> MMEGVKDFKQELLLVLPA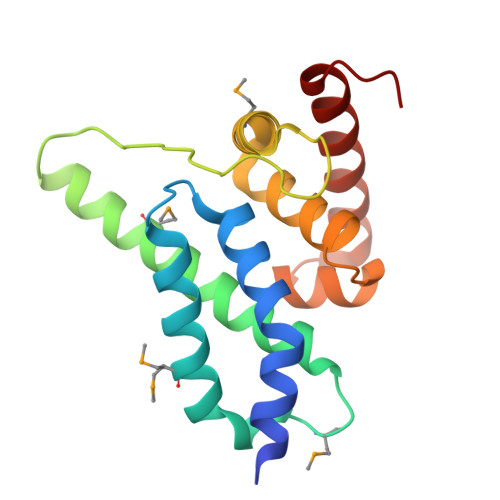LRAFAISLSSKHDKAEDLVQDTLMKAWAKQDSFEMGSNLKAWLFTILRNEFYSQMRKRGREVQDSDGVFIESVAIHPAQYGSLDLQDFKKALNMLSADQREAIILIGASGFSYEDAAAICGCAIGTIKSRVSRARNRLQELLKVDR> SNAMKNYYSSNPTFYLGIDCIIFGFNEGEISLLLLKRNFEPAMGEWSLMGGFVQKDESVDDAAKRVLAELTGLENVYMEQVGAFGAIDRDPGERVVSIAYYALININEYDRELVQKHNAYWVNINELPALIFDHPEMVDKAREMMKQKASVEPIGFNLLPKLFTLSQLQSLYEAIYGEPMDKRNFRKRVAEMDFIEKTDKIDKLGSKRGAALYKFNGKAYRKDPKFKL

In this study we identified and characterized a novel L-arabinose-responsive transcription factor found in the Bacteroides species, which belongs to the NrtR family of Nudix-related transcriptional regulators. The NrtR family transcription factors are characterized by an N-terminal Nudix hydrolase-like effector-binding domain and a C-terminal DNA-binding domain. In this work, genome-scale regulon inference using the comparative genomics approach revealed that the NrtR family AraR regulators in Bacteroides and Prevotella spp. control not only the L-arabinose catabolic operons, but also several other gene loci involved in the utilization of arabinose-containing polysaccharides. The predicted AraR-regulated operons are involved in the uptake and catabolism of L-arabinose and the decomposition of arabinose-containing polysaccharides (e.g., arabinan, arabinoxylan, pectic galactan) to oligosaccharides, their translocation into the periplasm, and further hydrolysis.

We determined the structures of full-length apo–BtAraR protein, its complex with a specific DNA duplex, and its complex with the L-arabinose effector. The solved structures provide a first view of the structural mechanism underlying the regulatory function of the L-arabinose-binding Nudix domain. The Nudix signature motif GX5-EX7REUXEEXGU (where U is a hydrophobic residue and X is any residue) is strictly conserved in all known active Nudix hydrolases, but it is impaired in the NrtR regulators of NAD metabolism, several of which are known to be enzymatically inactive. Similarly to NrtR regulators, the Nudix signature motif is not conserved in the AraR proteins from Bacteroidetes, where two or three glutamate residues are substituted with other amino acids. These observations suggest that AraR regulators are also enzymatically inactive and utilize their Nudix hydrolase-like domains for ligand binding.> MEPAGRFTKVAAAVADSVVTIESVSDQEGM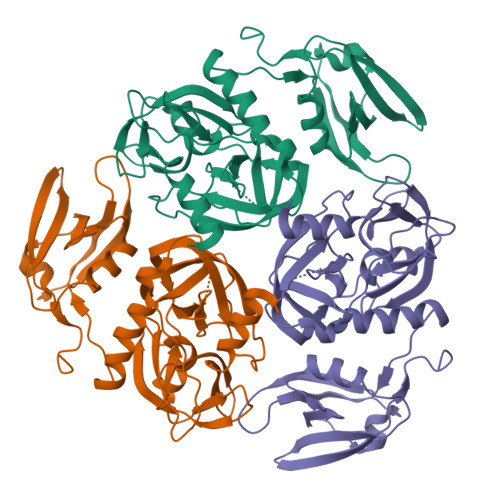QGSGVIVDGRGYIVTNNHVISEAANNPSQFKTTVVFNDGKEVPANLVGRDPKTDLAVLKVDNVDNLTVARLGDSSKVRVGDEVLAVGAPLGLRSTVTQGIVSALHRPVPLSGEGSDTDTVIDAIQTDASINHGNSGGPLIDMDAQVIGINTAGKSLSDSAAGLGFAIPVNEMKLVANSLIKDGKIVHPTLGISTRSVSNAIASGAQVANVKAGSPAQKGGILENDVIVKVGNRAVADSDEFVVAVRQLAIGQDAPIEVVREGRHVTLTVKPDPDSTLEHHHHHH>MKEKPAVEVRLDKWLWAARFYKTRALAREMIEGGKVHYNGQRSKPSKIVELNATLTLRQGNDERTVIVKAITEQRRPASEAAL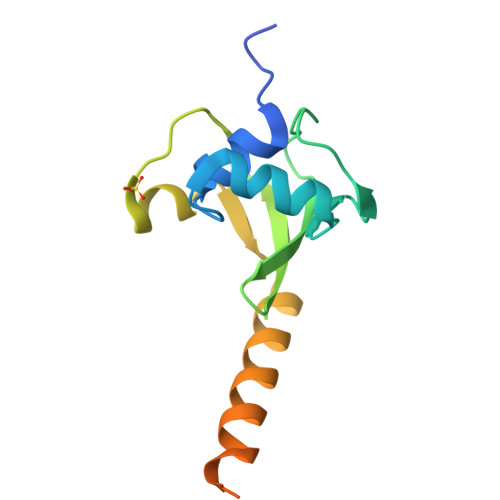LYEETAESVEKREKMALARKLNALTMPHPDRRPDKKERRDLLRFKHGDSE[2x]>MPLVLDLARPVSEEELRRLSELNPGYQWERSPEGRLWVSPTGGESGRRSLQLAYQLARWNEERGLGVVFDSSTGFKFPDGSILSPDAAFVERGAWEALSEAEREGFPPLAPKAVFEVRSASQDPEELRAKMGIYLRNGVLLGVLVDPYAR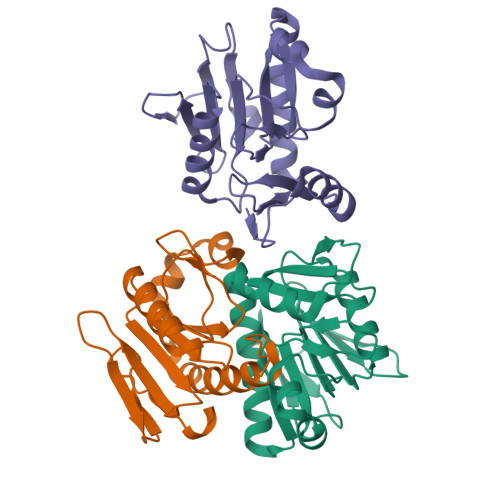AVEVFRPGKPPLRLEGVERVSLDPELPGFALSLPPLW[3x]> 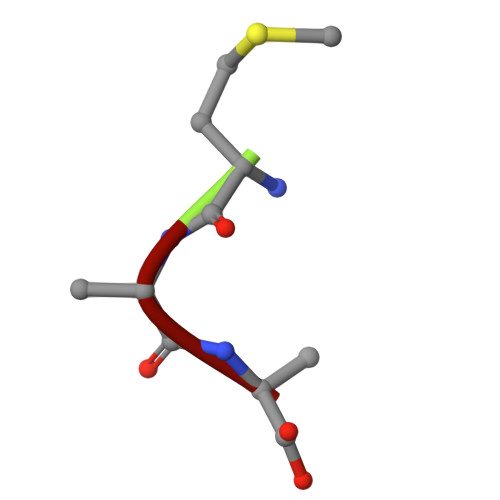MAA>IEMKPHPWFFGKIPRAKAEEMLSKQRHDGAFLIRESESAPGDFSLSVKFGNDVQHFKVLRDGAGKYFLWVVKFNSLNELVDYHR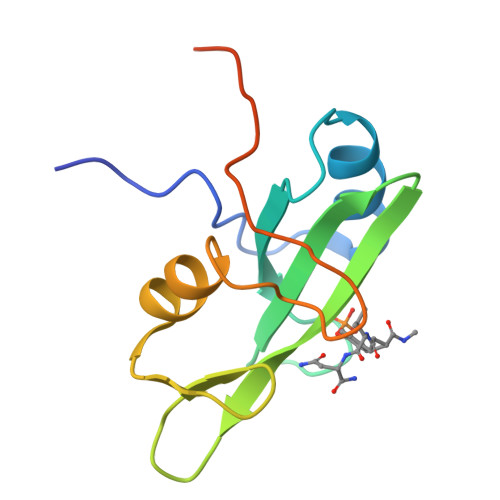STSVSRNQQIFLRDIEQVPQQPTYVQHHHHHH[2x]>ARNPITITPQFDCGATNSQQYVARSGDTLTKIAQEIYHDVVGVCDIARANNLADPNRIDAGTPYTIPINCQTYDRNSCL[4x]

The LysM effectors Mg1LysM and Mg3LysM, with one and three LysM domains, respectively, have been characterized from the Septoria tritici blotch pathogen of wheat, Z. tritici. Intriguingly, however, Mg1LysM was characterized as a functional homolog of Avr4 that protects hyphae against hydrolysis by host chitinases. The crystal structure of Mg1LysM from the Septoria blotch pathogen of wheat, Zymoseptoria tritici, revealed that chitin-induced dimerization of two Mg1LysM protomers through high affinity binding is required for hyphal protection against chitinases. Since Mg1LysM also forms ligand-independent homodimers, a supramolecular structure can be formed in which chitin-induced oligomerization of Mg1LysM ligand-independent homodimers form a contiguous Mg1LysM higher ordered structure that is anchored to the chitin in the fungal cell wall to prevent hydrolysis by host chitinases.

To this end, Mg1LysM was heterologously produced in the yeast Pichia pastoris and purified based on the presence of a His-FLAG affinity tag. The large Mg1LysM crystals that were finally obtained by micro-seeding techniques [31]belonged to the space group P 61 2 2. A native dataset was finally refined to a resolution of 2.41 Å with an Rwork and Rfree of 17.96% and 22.03%, respectively. The structure model comprises in total four copies of the complete mature protein sequence except for the first amino acid after the signal peptide for chains A to C and the first two amino acids after the signal peptide for chain D, and one carbohydrate molecule per asymmetric unit (a.u.). The compact LysM structure is stabilized by two disulfide bridges between Cys44 and Cys78, and between Cys13 and Cys70. In addition to the single LysM domain, Mg1LysM comprises a relatively long N-terminal tail that contains a short β-strand. The four Mg1LysM monomers within the a.u. form two pairs of homodimers that are each very tightly packed. In addition, the crystal structure revealed that the N-terminal 12 amino acid tails of the homodimer run anti-parallel and form a small but stable β-sheet (5ITI7 of each chain) that is stabilized by clustering of all four isoleucine side-chain residues and by threonine-threonine sidechain hydrogen bonding, potentially strengthening the homodimer. The latter hypothesis is further supported by the formation of two additional salt bridges formed between Arg2 of one subunit and Asp12 of the other one.> MGSDKIHHHHHHMVMEYELRTPLVKDQILKLKVGDVVYITGEIFTARDEAHARALEWMEEGKELPFSFDKGVVYHCGPLVKKNDEWRVVSAGPTTSARMNPFTPKILEKVECMGIIGKGGMSEEVVEAMRGKAAYFAFTGGAGALAAMSIKKVKGVVWEDLGMPEAVWLLEVERFGPCIVAIDAHG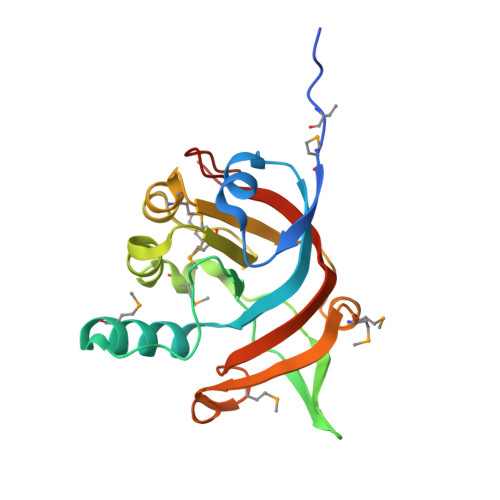NSLYRR>[2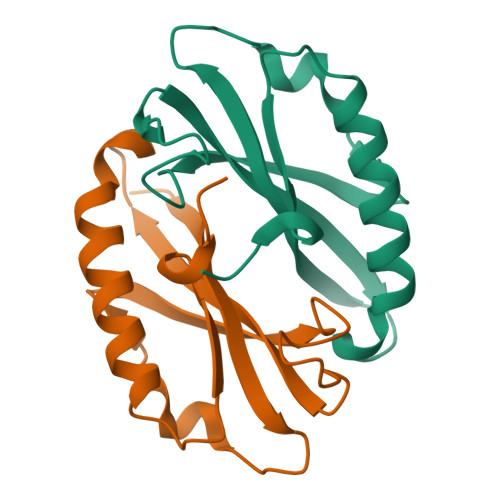x]MQAVRLFQGYMWHPRALALDLKALLPGEVAGARLLWDEVPPPTPFFEDGTPTHTQRFYQLTLLVLTEEPPEALKPLAEEAAEALGEVLEGLPPEVGWLLLEDLRPL> ADPGTPGEAEGPACPAACVCSYDDDADELSVFCSSRNLTRLPDGVPGGTQALWLDGNNLSS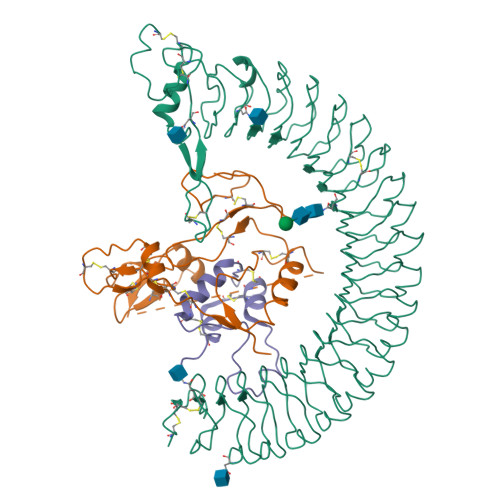VPPAAFQNLSSLGFLNLQGGQLGSLEPQALLGLENLCHLHLERNQLRSLALGTFAHTPALASLGLSNNRLSRLEDGLFEGLGSLWDLNLGWNSLAVLPDAAFRGLGSLRELVLAGNRLAYLQPALFSGLAELRELDLSRNALRAIKANVFVQLPRLQKLYLDRNLIAAVAPGAFLGLKALRWLDLSHNRVAGLLEDTFPGLLGLRVLRLSHNAIASLRPRTFKDLHFLEELQLGHNRIRQLAERSFEGLGQLEVLTLDHNQLQEVKAGAFLGLTNVAVMNLSGNCLRNLPEQVFRGLGKLHSLHLEGSCLGRIRPHTFTGLSGLRRLFLKDNGLVGIEEQSLWGLAELLELDLTSNQLTHLPHRLFQGLGKLEYLLLSRNRLAELPADALGPLQRAFWLDVSHNRLEALPNSLLAPLGRLRYLSLRNNSLRTFTPQPPGLERLWLEGNPWDCGCPLKALRDFALQNPSAVPRFVQAICEGDDCQPPAYTYNNITCASPPEVVGLDLRDLSEAHFAPC;> GASSAGLGPVVRCEPCDARALAQCAPPPAVCAELVREPGCGCCLTCALSEGQPCGIYTERCGSGLRCQPSPDEARPLQALLDGRGLCVNASAVSRLRAYLLPAPPAPGNASESEEDRSAGSVESPSVSSTHRVSDPKFHPLHSKIIIIKKGHAKDSQRYKVDYESQSTDTQNFSSESKRETEYGPCRREMEDTLNHLKFLNVLSPRGVHIPNCDKKGFYKKKQCRPSKGRKRGFCWCVDKYGQPLPGYTTKGKEDVHCYSMQSK;> GPETLCGAELVDALQFVCGDRGFYFNKPTGYGSSSRRAPQTGIVDECCFRSCDLRRLEMYCAPLKPAKSA> GSEFVKEHDWKKCDQSGFCRRNRAYADHALSAISWESPYKIAPETGSFKDGQYQAIILKTINDHGETVRLPLTVSFLESGTARVTIDEEKRQKGEIELRHDSKARKERYNEAEQWVIVGGMTLDKGAKVDYEDKTQMTVKYGPSSKFEATIKFAPFSIDFKRDGASHIKFNDQGLLNIEHWRPKIDPPPEPEKKEGEQQPDKKEEAPREDDSTWWEESFGGNTDSKPRGPESVGLDISFVGYEHVFGIPSHASPLSLKQTRGGEGNYNEPYRMYNADVFEYILDSPMTLYGSIPFMQAHRKDSSVGIFWLNAAETWVDITKGKDSKNPLALGVKSKITTRTHWFSESGLLDVFVFLGPTPKDIISKYAELTGTTAMPQEFSLGYHQCRWNYVSDEDVKDVDRKMDKFNMPYDVIWLDIEYTDEKKYFTWDKHSFKDPIGMGKQLEAHGRKLVTIIDPHIKNTNNYPVVDELKSKDLAVKTKDGSIFEGWCWPGSSHWIDAFNPAAREWWKGLFKYDKFKGTMENTFIWNDMNEPSVFNGPEVTMPKDNLHHGNWEHRDVHNLNGMTFQNATYHALLSRKPGEHRRPFVLTRAFFAGSQRLGAMWTGDNTADWGYLKASIPMVLSQGIAGFPFAGADVGGFFGNPDKDLLTRWYQTGIFYPFFRAHAHIDARRREPYLTGEPYNTIIAAALRLRYSLLPSWYTAFRHAHLDGTPIIKPMFYTHPSEEAGLPIDDQFFIGNTGLLAKPVTDKDRTSVDIWIPDSEVYYDYFTYDIISAAKSKTATLDAPLEKIPLLMRGGHVFARRDIPRRSSALMKWDPYTLVVVLGNDRKAEGDLYVDDGDSFDYEKGQYIHRRFIFDANTLTSADYEGRDDASIKEGEWLKKMRTVNVEKIIVVGAPAAWKGKKTVTVESEGKTWAAAIEYNPAEKSRAAFAVVKKVGVRVGADFKIVFG

Glucosidase I removes the outermost α1,2-linked glucose from the D1 branch, and then glucosidase II (GII) trims second and third α1,3-linked glucose residues by catalyzing hydrolyses at the Glc-α1,3-Glc and Glc-α1,3-Man glycosidic linkages. Here we performed an X-ray crystallographic study of GIIα to elucidate its substrate recognition mechanism. The overall structure of GIIα is composed of four major domains and three subdomains: N-terminal domain (residues 31–384), subdomain B1 (residues 207–256), β8α8 barrel domain (residues 385–737), subdomain B2 (residues 484–526), subdomain B3 (residues 559–581), proximal C-terminal domain (residues 738–823), and distal C-terminal domain (residues 824–977). Taken together, our structural data revealed that GIIα can recognize two kinds of glucosylated substrates, Glc-α1,3-Glc and Glc-α1,3-Man, via a bilocular substrate-binding pocket with a tolerant +1 subsite.

We expressed the recombinant GIIα (residues 31–977) in Escherichia coli and crystallized it by the hanging-drop vapor diffusion method. The crystal belongs to space group R32 with one molecule per asymmetric unit. The final model of GIIα refined to 1.40 Å resolution has an Rwork of 15.4% and Rfree of 17.5%. The tris(hydroxymethyl)aminomethane (Tris) molecule derived from the crystallization reagent, also known as an α-glucosidase inhibitor, was accommodated in the putative active-site pocket located at the center of β8α8 barrel domain. The Tris molecule was bound to the pocket in the 1.40-Å-resolution crystal structure. Similar to DNJ, it interacted with Asp443, Asp556, Arg617, Asp633, and His691 through hydrogen bonds. The α1 helix covers a β sheet comprising β12, β17, and β18, and, the preceding 11-residue-long segment is accommodated in the putative active site pocket of β8α8 barrel domain, suggesting its involvement in substrate binding. A unique subdomain (termed B1) is found in the N-terminal domain of GIIα but not in the other GH31s. In subdomain B1, residues 215–235 are completely disordered, suggesting its flexible nature. In this domain, a continuous twisted β strand (β43) connects the β sheets with β42 and β44, forming a β-barrel-like structure. These C-terminal domains appear to be responsible for the stabilization of the β8α8 barrel domain rather than for substrate binding, given that no interactions between these C-terminal domains and the active-site pocket were observed.> ECVTQLLKDTCFEGGDITTVFTPSAKYCQVVCTYHPRCLLFTFTAESPSEDPTRWFTCVLKDSVTETLPRVNRTAAISGYSFKQCSHQISACNKDIYVDLDMKGINYNSSVAKSAQECQERCTDDVHCHFFTYATRQFPSLEHRNICLLKHTQTGTPTRITKLDKVVSGFSLKSCALSNLACIRDIFPNTVFADSNIDSVMAPDAFVCGRICTHHPGCLFFTFFSQEWPKESQRNLCLLKTSESGLPSTRIKKSKALSGFSLQSCRHSIPVFCHSSFYHDTDFLGEELDIVAAKSHEACQK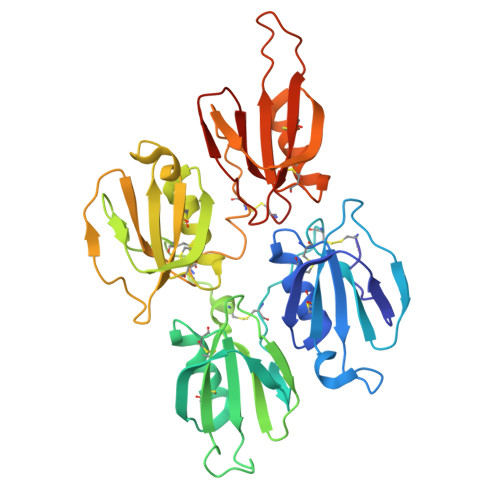LCTNAVRCQFFTYTPAQASCNEGKGKCYLKLSSNGSPTKILHGRGGISGYTLRLCKM> MPPKQTKVVASRKTVMPISRAGRAQIRRKDSNTQNNMNDQGMEDEEIDQQREGMKNQYEQLTAQELNEDMPSKMLEPKNPQAPKNITVYDYYTRKFKTDELVDQMIVHFSMDGDYIWKESNEYKTQEEIRDTKKALIKEAMRKQESEEPGANHDEEAIKQTLRNKFNYNTRECQTINPSIRERGVSTEPPPSDTICGNITQWEIFDAYYAEIMKDHQIENKKKKEVDQDKKQDQSMYSTSFKRCCKIMERMVVQNDQEDKYHDYRYYWSQGDNLEAGKNEGHLLPIWRFSNEKQRKKNVTSICWNPLYPDLFAVSLGSYDFTKQRMGLICLYSLKNTTHPEYAFNCEAGVMCLDFHPKSAALLAVGLYDGTVLVYDIRNKHKKPIYQSTVRNQKHTDPVWQVKWNPDTSKNYNFYSISSDGRVMNWILMKNKLEPEEVILLRLVGKNEEESTLIGLACGLCFDFNKFEPHIFLVGTEEGKIHKCSRAYSGQYQETYNGHLLAVYKVKWNNFHPRTFISASADWTVRIWDSKYTSQIICFDLSMMVVDAVWAPYSSTVFACATMDKVQVYDLNVDKLNKLAEQKIVKQPKLTNLSFNYKDPILLVGDSHGGVTLVKLSPNLCKS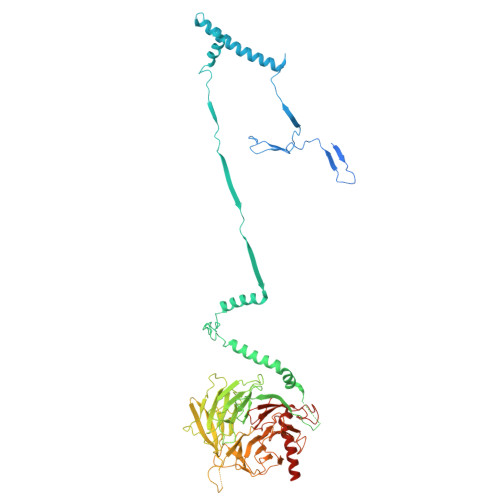GPEIKQTEDKKAMEEFKNVKIEDYEREKMENLLAVVSKWEREDA The K+ uptake system KtrAB is essential for bacterial survival in low K+ environments. The activity of KtrAB is regulated by nucleotides and Na+. The KtrAB system is composed of the transmembrane KtrB dimer, each containing four structurally similar domains (D1~D4) arranged around a four-fold pseudosymmetry axis normal to the cell membrane, and the regulatory KtrA octamer (tetramer of homodimer) with a ring-like structure, known as the RCK gating ring. ATP binding to KtrA octamer activates K+ flux activity of KtrB, whereas ADP binding inactivates it.

Mg2+-added and Mg2+-free ATP-BsKtrAB cryo-EM structures (Structure I and Structure II) are virtually identical with an r.m.s.d. of 0.30 Å over 2104 Cα atoms. A clear region of unassigned cryo-EM density between the two adjacent ATPs at the intra-dimer interface was observed in Structure I. To minimize the uncertain effects that Mg2+ may cause on the structure of BsKtrAB (Structure I), we hereafter used Mg2+-free ATP-BsKtrAB (Structure II) in comparison with ADP-BsKtrAB (Structure III) for the following structural analysis.

>[8x]MGRIKNKQFAVIGLGRFGGSICKELHRMGHEVLAVDINEEKVNAYASYATHAVIANATEENELLSLGIRNFEYVIVAIGANIQASTLTTLLLKELDIPNIWVKAQNYYHHKVLEKIGADRIIHPEKDMGVKIAQSLSDENVLNYIDLSDEYSIVELLATRKLDSKSIIDLNVRAKYGCTILAIKHHGDICLSPAPEDIIREQDCLVIMGHKKDIKRFENEGM;>MTLQKDKVIKWVRFTPPQVLAIGFFLTIIIGAVLLMLPISTTKPLSWIDALFTAASATTVTGLAVVDTGTQFTVFGQTVIMGLIQIGGLGFMTFAVLIVMILGKKIGLKERMLVQEALNQPTIGGVIGLVKVLFLFSISIELIAALILSIRLVPQYGWSSGLFASLFHAISAFNNAGFSLWPDNLMSYVGDPTVNLVITFLFITGGIGFTVLFDVMKNRRFKTFSLHTKLMLTGTLMLNAIAMLTVFILEYSNPGTLGHLHIVDKLWASYFQAVTPRTAGFNSLDFGSMREGTIVFTLLLMFIGAGSASTASGIKLTTFIVILTSVIAYLRGKKETVIFRRSIKYPIIIKALAVSVTSLFIVFLGIFALTITEQAPFLQIVFETFSAFGTVGLTMGLTPELTTAGKCIIIVIMFIGRIGPLTFVFSFAKTEQSNIRYPDGEVFTG[4x]Basement membranes are extracellular structures of epithelia and endothelia that have collagen IV scaffolds of triple α-chain helical protomers that associate end-to-end, forming networks. At the C-termini, interactions occur between the trimeric NC1 domains of two protomers, forming a hexamer of these domains reinforced by sulfilimine cross-links. Recent studies in one of our laboratories revealed that the NC1 domains function as recognition modules, directing the selection and assembly of α-chains into protomers and networks.

The asymmetric unit included two subunits. Following application of the crystal symmetry, each subunit formed a protomer with fourfold molecular symmetry. One of these protomers was isolated and the other generated a homo-octamer (α2NC1homo). α2NC1homo resembled a canonical hexamer, except for an increase in the number of subunits to four per protomer, enlarging the equatorial circumference somewhat (∼70 Å diameter) and widening the central tunnel (∼30 Å). Therefore, the two self-assembled noncanonical structures of α2NC1 or α4NC1 subunits may lack some structural elements that are present in the canonical trimeric protomers that could intrinsically restrict the formation of protomers with more than three subunits. The comparison between the structure of the α2NC1 domain in its noncanonical homohexamer and the same domain in α121NC1 (α2NC1α121) revealed that there are conformational differences that might explain the greater number of subunits. The presence of an isolated tetrameric protomer that is not associated into an octamer in the α2NC1homo crystal is structural evidence of weakened interactions across the equatorial plane. Our findings of noncanonical assemblies for α2NC1 and α4NC1 homo-oligomers and the structural changes observed in the chains forming these noncanonical protomers in comparison to α2NC1α121 and to the chains in α1NC1homo, α3NC1homo and α5NC1homo could imply that chain folding is closely related to protomer assembly. It is unlikely that α2NC1homo and α4NC1homo could represent stable physio­logical assemblies, but the structures of the individual chains in these noncanonical oligomers might provide a frozen glimpse of transient conformational states in the process of NC1 folding and hexamer building.

>[2x]SVSIGYLLVKHSQTDQEPMCPVGMNKLWSGYSLLYFEGQEKAHNQDLGLAGSCLARFSTMPFLYCNPGDVCYYASRNDKSYWLSTTAPLPMMPVAEDEIKPYISRCSVCEAPAIAIAVHSQDVSIPHCPAGWRSLWIGYSFLMHTAAGDEGGGQSLVSPGSCLEDFRATPFIECNGGRGTCHYYANKYSFWLTTIPEQSFQGSPSADTLKAGLIRTHISRCQVCMKNL>[6x]GAMGSTVGLTA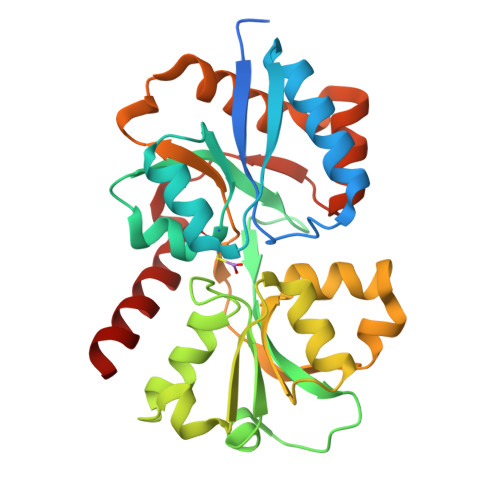LKVSGETLSEPMRPGVIRFGLTPVFLSNDLEVLDELQAYLTQAVGQEVQLITQRTYQEVTALLVSGNLEAAWICGYPFMKFRDELDLVATPLWRGKPVYQSYLIVGRDRDIAGFEDCQGDIHAFSDPDSNSGYLVTKTYLAERGVSEEGFFRKSFFTYGHRNVIRAVASGLADSGSVDGYVWEVMKTTEPELVAKTRVLVKSGWHGFPPVAAAAGQRKSQAVARIRSALLDMNQEVLGRSVLTRLQLDGFVETTAESYDSIAANMERVRRLG>SFWGWLNAVFNKVDHDRIRDVGPDRAASEWLLRCGAMVRYHGQQRWQKDYNHLPTGPLDKYKIQAIDATDSCIMSIGFDHMEGLQYVEKIRLCKCHYIEDGCLERLSQLENLQKSMLEMEIISCGNVTDKGIIALHHFRNLKYLFLSDLPGVKEKEKIVQAFKTSLPSLELKLDLK[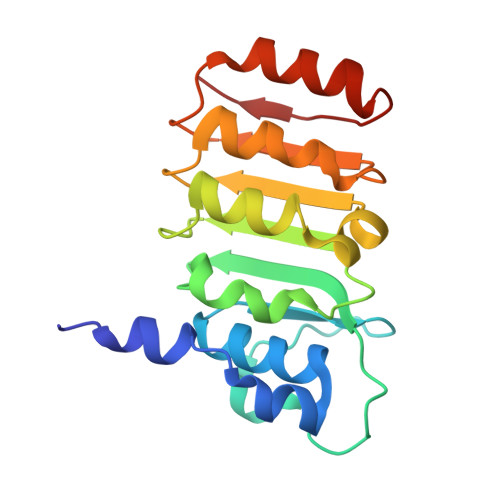4x]>[4x]GVQLTAAQELMIQQLVAAQLQCNKRSFSDQPKVTPWPLGADPQSR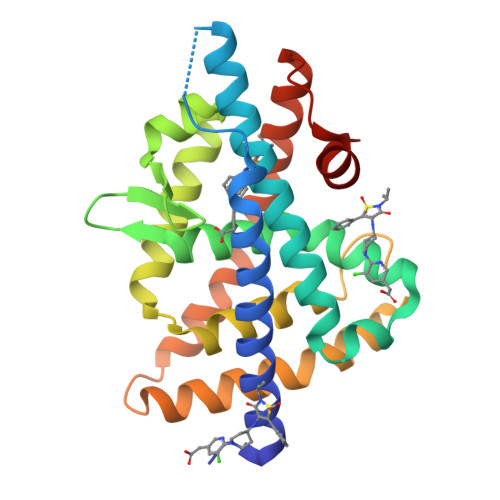DARQQRFAHFTELAIISVQEIVDFAKQVPGFLQLGREDQIALLKASTIEIMLLETARRYNHETECITFLKDFTYSKDDFHRAGLQVEFINPIFEFSRAMRRLGLDDAEYALLIAINIFSADRPNVQEPGRVEALQQPYVEALLSYTRIKRPQDQLRFPRMLMKLVSLRTLSSVHSEQVFALRLQDKKLPPLLSEIWDVHE> CCGGGT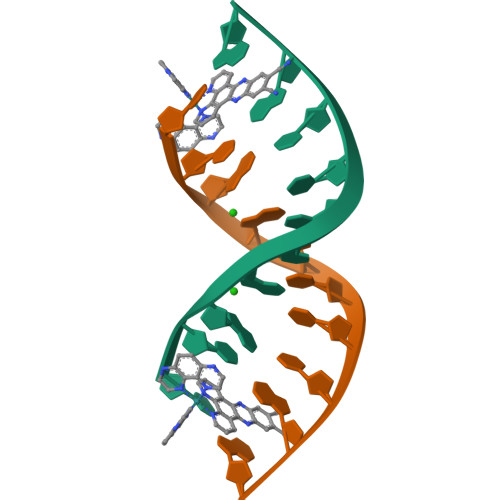CCGG;> CCGGACCCGG>MSPCGYYSKWRNRDRPEYRRNLRFRRFFSSIHPNAAAGSGFNGPGVFITSVTGVWLCFLCIFSMFVTAVVSVSPSSFYESLQVEPTQSEDITRSAHLGDGDEIREAIHKSQDAETKPTFYVCPPPTGSTIVRLEPPRTCPDYHLGKNFTEGIAVVYKENIAAYKFKATVYYKDVIVSTAWAGSSYTQITNRYADRVPIPVSEITDTIDKFGKCSSKATYVRNNHKVEAFNEDKNPQDMPLIASKYNSVGSKAWHTTNDTYMVAGTPGTYRTGTSVNCIIEEVEARSIFPYDSFGLSTGDIIYMSPFFGLRDGAYREHSNYAMDRFHQFEGYRQRDLDTRALLEPAARNFLVTPHLTVGWNWKPKRTEVCSLVKWREVEDVVRDEYAHNFRFTMKTLSTTFISETNEFNLNQIHLSQCVKEEARAIINRIYTTRYNSSHVRTGDIQTYLARGGFVVVFQPLLSNSLARLYLQELVRENTNHSPQKHPTRNTRSRRSVPVELRANRTITTTSSVEFAMLQFTYDHIQEHVNEMLARISSSWCQLQNRERALWSGLFPINPSALASTILDQRVKARILGDVISVSNCPELGSDTRIILQNSMRVSGSTTRCYSRPLISIVSLNGSGTVEGQLGTDNELIMSRDLLEPCVANHKRYFLFGHHYVYYEDYRYVREIAVHDVGMISTYVDLNLTLLKDREFMPLQVYTRDELRDTGLLDYSEIQRRNQMHSLRFYDIDKVVQYDSGTAIMQGMAQFFQGLGTAGQAVGHVVLGATGALLSTVHGFTTFLSNPFGALAVGLLVLAGLVAAFFAYRYVLKLKTSPMKALYPLTTKGLKQLPEGMDPFAEKPNATDTPIEEIGDSQNTEPSVNSGFDPDKFREAQEMIKYMTLVSAAERQESKARKKNKTSALLTSRLTGLALRNRRGYSRVRTENVTGV[3x]

A cooperative assembly of glycoproteins composed of the trimeric gB and the heterodimer gH-gL constitutes the core herpesvirus fusion complex. Due to structural similarities with viral fusogens of vesicular stomatitis virus (VSV) G protein and baculovirus gp64, gB has been designated a type III fusogen. As for other herpesviruses, VZV employs gB and gH-gL for virion entry fusion. Unlike the closely related herpes simplex virus (HSV) gB orthologues, the mature glycosylated form of VZV gB (~130kDa) is cleaved into two fragments (~69kDa and ~73kDa) at the 491RSRR494 furin recognition site.

Structures of native, full-length VZV gB (cryo-EM; 3.9Å) and the VZV gB ectodomain (X-ray crystallography; 2.4Å) were determined in the absence of bound antibodies to define the structure of the N-terminal region (amino acids (aa)72-114), which was found to be a part of DIV but flexible and not fully resolved by cryo-EM or X-ray crystallography. Full-length gB was visible as rod-like particles ~20 nm in length in vitreous ice on ultrathin carbon film supported on lacey carbon EM grids. The cryo-EM structure of the native, full-length gB ectodomain was resolved at near atomic resolution (3.9Å) with an architecture resembling the postfusion form resolved for herpesvirus gB orthologues. Cryo-EM 2D class averages generated from 349,207 particles revealed four globular regions of gB, three in the ectodomain and one in the CTD. The gB domains, DI-DV, were apparent in the cryo-EM map of the gB trimer constrained to a 3-fold (C3) axis of symmetry. In contrast to the ectodomain, the cryo-EM map resolution of the CTD, including the MPR, transmembrane (TM) and gBcyt, was >7.0Å due to extensive flexibility in the CTD that was apparent from the 2D class averages. The Cα backbone could not be traced for aa72-114 in either the cryo-EM or X-ray crystallography datasets. Importantly, the detection of peptides corresponding to aa94-114 verified the presence of the N-terminus in full-length gB and supports flexibility as the reason for failure to resolve this region in the gB structures. The gB cryo-EM structures did not differ in the presence or absence of 93k and SG2 Fabs, indicating that the gB ectodomain in its post fusion form was not altered by antibody binding. Comparison of the cryo-EM map derived model of native gB purified from VZV infected cells with the gB crystal structure demonstrated that the W180G and Y185G substitutions did not affect fusion loop topology.> SLSCRPPMVKLVCPADNLRAEGLECTKTCQNYDLECMSMGCVSGCLCPPGMVRHENRCVALERCPCFHQGKEYAPGETVKIGCNTCVCQDRKWNCTDHVCDATCSTIGMAHYLTFDGLKYLFPGECQYVLVQDYCGSNPGTFRILVGNKGCSHPSVKCKKRVTILVEGGEIELFDGEVNVKRPMKDETHFEVVESGRYIIL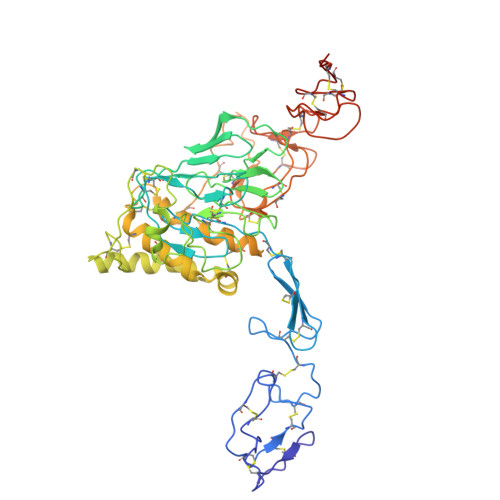LLGKALSVVWDRHLSISVVLKQTYQEKVCGLCGNFDGIQNNDLTSSNLQVEEDPVDFGNSWKVSSQCADTRKVPLDSSPATCHNNIMKQTMVDSSCRILTSDVFQDCNKLVDPEPYLDVCIYDTCSCESIGDCACFCDTIAAYAHVCAQHGKVVTWRTATLCPQSCEERNLMENGYECMWRYNSCAPACQVTCQHPEPLACPVQCVEGCHAHCPPGKILDELLQTCVDPEDCPVCEVAGRRFASGKKVTLNPSDPEHCQICHCDVVNLTCEACQEPGGLVVPPHHHHHH> MFDQLAVFTPQGQVLYQYNCLGKKFSEIQINSFISQLITSPVTRKESVANANTDGFDFNLLTINSEHKNSPSFNALFYLNKQPELYFVVTFAEQTLELNQETQQTLALVLKLWNSLHLSESILKNR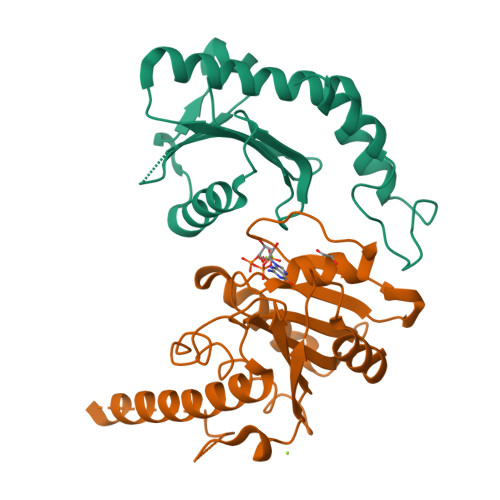QGQNEKNKHNYVDILQGIEDDLKKFEQYFRIK;> GSHMGIKQKSYQPSIIIAGPQNSGKTSLLTLLTTDSVRPTVVSQEPLSAADYDGSGVTLVDFPGHVKLRYKLSDYLKTRAKFVKGLIFMVDSTVDPKKLTTTAEFLVDILSITESSCENGIDILIACNKSELFTARPPSKIKDALESEIQKVIERRKKSLNEVERKINEEDYAENTLDVLQSTDGFKFANLEASVVAFEGSINKRKISQWREWIDEKL>ASDANINLSSEKQLIKGFGGINHPAWIGDLTAAQRETAFGNGQNQLGFSILRIYVDDNRNNWYREVATAKRAIEQGALVFASPWNPPSDMVETFNRNGASAKRLKYDKYAAYAQHLNDFVTFMKNNGVDLYAISVQNEPDYAHDWTWWTPQEILRFMKENAGSIQGTRVMAPESFQYLKNISDPIL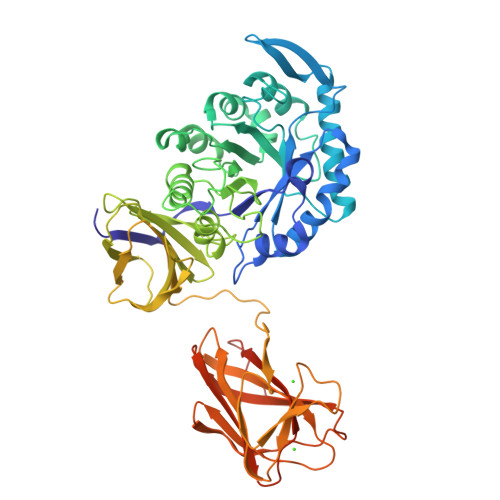NDPQALANMDILGAHTYGTQIKDFAYPLFKQKGAGKELWMTEVYVPNSDNNSADRWPEALDVSYHMHNAMVEGDFQAYVWWYIRRQYGPMKEDGTISKRGYNMAHFSKFVRPGYVRVDATKNPDTNTYVSAYKGDNKVVIVAINRGTSAASQRFVLQNGNASTVSSYVTDSSRNLASLAPINVSNGAFTAQLPAQSVTTFVANLSGGNSGGGNVNTGTTYEAETGTTLTDAVVETLYPGYTGSGYVNFNAYTNSAIEWNAINNMTTGTKNVKFRYALESGTRNLDIYVNGTKVLSNEPFTETGSWSTWGEKTIQVAMNSGVNTLRIVTTGTEGPNMDNITVTASAKGELNSKLEGKPIPNPLLGLDSTRTGHHHHHH[8x]> GHMKVTSVAMPSYIGSSLEFTKNNLIQIVGIKEANIEVVEVTTAPAGSVEGMVVEQSPRAGEK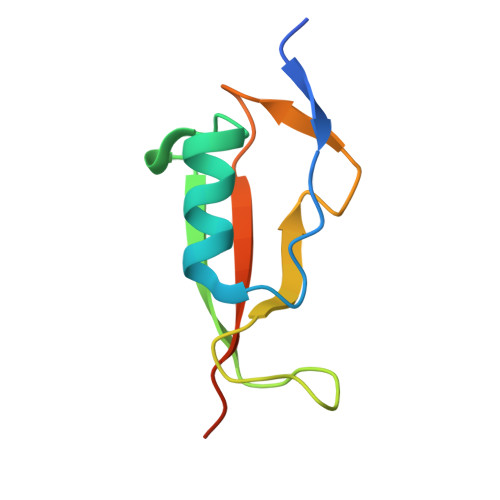VDLNKTRVKISIYKPKTTSATP>MTIGIDKISFFVPPYYIDMTALAEARNVDPGKFHIGIGQDQMAVNPISQDIVTFAANAAEAILTKEDKEAIDMVIVGTESSIDESKAAAVVLHRLMGIQPFARSFEIKEACYGATAGLQLAKNHVALHPDKKVLVVAADIAKYGLNSGGEPTQGAGAVAMLVASEPRILALKEDNVMLTQDIYDFWRPTGHPYPMVDGPLSNETYIQSFAQVWDEHKKRTGLDFADYDALAFHIPYTKMGKKALLAKISDQTEA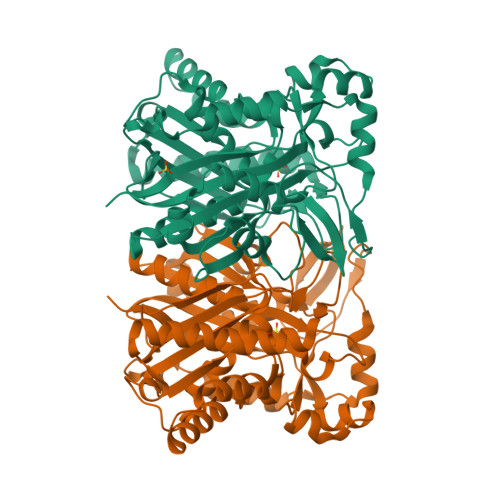EQERILARYEESIIYSRRVGNLYTGSLYLGLISLLENATTLTAGNQIGLFSYGSGAVAEFFTGELVAGYQNHLQKETHLALLDNRTELSIAEYEAMFAETLDTDIDQTLEDELKYSISAINNTVRSYRN[2x]>MIIIGIDEAGRGPVLGPMVVCAFAIEKEREEELKKLGVKDSKELTKNKRAYLKKLLENLGYVEKRILEAEEINQLMNSINLNDIEINAFSKVAKNLIEKLNIRDDEIEIYIDACSTNTKKFEDSFKDKIEDIIKERNLNIKIIAEHKADAKYPVVSAASIIAKAERDEIIDYYKKIYGDIGSGYPSDPKTIKFLEDYFKKHKKLPDIARTH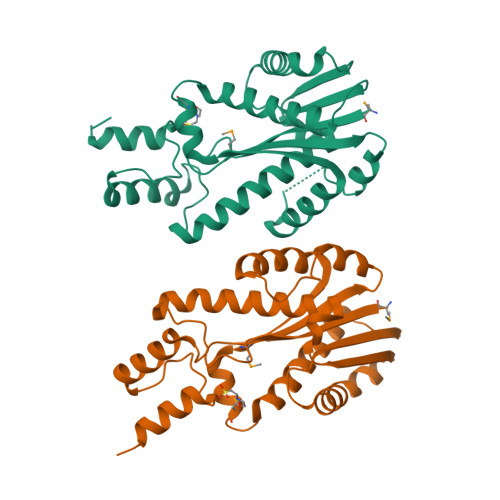WKTCKRILDKSKQTKLIIE[2x]> GPLGSPEFDCHLSDMLQQLHSVNASKPSERGLVRQEEAEDPACIPIFWVSKWVDYSDKYGLGYQLCDNSVGVLFNDSTRLILYNDGDSLQYIERDGTESYLTVSSHPNSLMKKITLLKYFRNYMSEHLLKAGANITPREGDELARLPYLRTWFRTRSAIILHLSNGSVQINFFQDHTKLILCPLMAAVTYIDEKRDFRTYRLSLLEEYGCCKELASRLRYARTMVDKLLSSR;> XLDP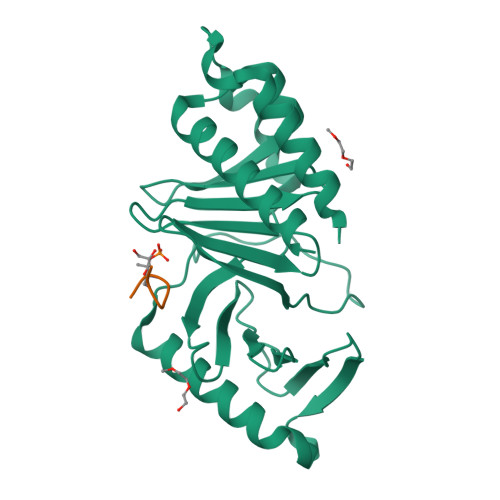PLHSTAX6-CHLORO-4-(CYCLOHEXYLSULFANYL)-3-PROPYLQUINOLIN-2(1H)-ONE | C18 H22 Cl N O S | 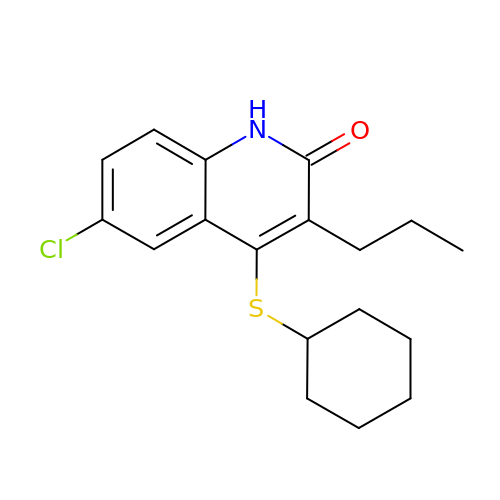CLKFNGKDJYMUPK-UHFFFAOYSA-N(1R,2R,3S,4S)-3-[4-(4-fluorophenyl)piperazine-1-carbonyl]bicyclo[2.2.1]heptane-2-carboxylic acid | C19 H23 F N2 O3 | 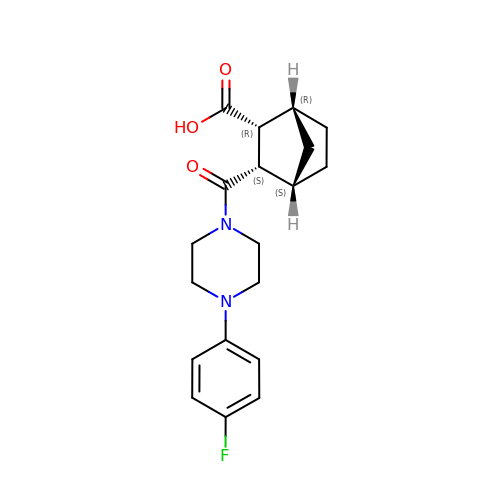IGLAQRKZPMAAST-UWWPHRKUSA-N> MSHKR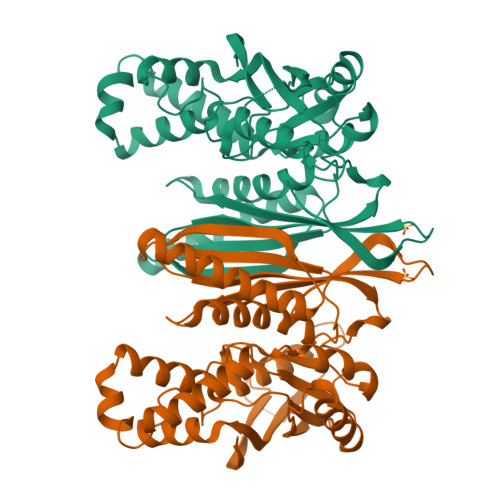PQSSAGESNGAVDLKTPRFDPVSLGLPAEFQLTDYTRLKGCSCKLPQPKLLALLQELSATPGQKDVGMDCSIVPLHHTNSKGEALFLVSTTDFFFPSVSDPFLQGQIGAANVLSDLYSMGIPDCDTMLMLLAASTEMDEHERLITTREIMKGFAERARLATTTVTGGQTVMNPWPLIGGVAMAVVSEAEMVRPTGLLCAGDILVLTKPLGCQVAVNLKQWLLRPSPLYEEAIAGHISPEEIEELYNMATDSMRRLNREGARLMRKHGAHGATDVTGFGILGHANNFGAAQAVGDAPRSLCLVLERLPMFKTAVAASKQMNDKYRLLEGYSAETSGGLLVAFPSTTAAAAFCAELTAVDGGCPSWIVGHVEDRATNAVDGVYARLKDGYEIVEV Homoserine dehydrogenase (HseDH, EC 1.1.1.3) is a key enzyme in the biosynthetic pathway from aspartate to homoserine (Hse), which is a common precursor for the synthesis of three amino acids, methionine, threonine and isoleucine in plants and microorganisms. The third enzyme in the pathway, HseDH, catalyzes the NAD(P)H-dependent reduction of Asa to Hse. In the present study, we expressed that gene, which encoded a HseDH homolog, characterized the enzyme produced and revealed the enzyme to be a highly thermostable HseDH. Each monomer consisted of three domains: a nucleotide-binding domain (residues 1–139 and 297–315), a dimerization domain (140–160 and 266–293) and a substrate-binding domain (residues 161–265).

The structure of substrate-free P. horikoshii HseDH was determined using molecular replacement and refined at a resolution of 2.30 Å. The asymmetric unit consisted of one homodimer with a solvent content of 70.1%, which corresponded to a Matthews coefficient11 of 4.1 Å3 Da–1. The model of the dimer contained the ordered residues (1-319) in each subunit, two NADPH molecules (see below), five 2-methyl-2,4-pentanediol (MPD) molecules, two Na atoms and 212 water molecules. Our initial electron density map for the substrate-free P. horikoshii HseDH showed an extra density within the nucleotide-binding site and, after construction and refinement of the peptide chain, an NADP(H) molecule could be modeled into that density. No cofactor was present during crystal growth, but this molecule may have originated in the E. coli cells and was then retained throughout the protein purification. On the other hand, the mass of NADP was not detected in P. horikoshii HseDH. These results demonstrate that the molecule bound to P. horikoshii HseDH is NADPH. The electron density corresponding to the NADPH bound within the nucleotide-binding site of P. horikoshii HseDH was very clear, enabling us to place the ligand with reasonable accuracy. By contrast, the C2 phosphate group (O1X, O2X, and O3X) of the adenine ribose is tightly held at its position through interactions with the side chain and backbone N atom of Arg40, the side chain of Lys57, and via a water molecule (W4), the backbone O atom of Gly61. The C2 phosphate is tightly held in position through five surrounding hydrogen bonds in the wild-type enzyme. Given that no substantive difference in the domain organization of the two enzymes was found, these observations suggest that the larger number of interactions around the C2 phosphate of the cofactor strengthen the affinity of wild type HseDH for NADP, making the binding too tight to utilize NADP as the cofactor. The two nearly identical subunits (root-mean-square deviation (r.m.s.d.) = 0.35 Å) were closely associated mainly through hydrophobic interactions around α14, β14 and the C-terminal region (residues 314–318) in both subunits.

>MNHKVHHHHHHIEGRHMKVNISIFGFGTVGRALAEIIAEKSRIFGVELNVISITDRSGTIWGDFDLLEAKEVKESTGKLSNIGDYEVYNFSPQELVEEVKPNILVDVSSWDEAHEMYKVALGEGISVVTSNKPPIANYYDELMNLAKENNAGIFFESTVMAGTPIIGVLRENLLGENIKRIDAVVNASTTFILTKMSEGKTLDDAIEEAKSLGILEEDPSKDIDGIDAYYKAKILHWVSYGEPPEEEERLGIREVRDARNVRLVAQVSKGKISVKPRKLSSDNPLLVEGVQNAAVIRTNNLGEVILKGPGGGGRVTASGVFTDIIKATLKFPNLR[2x]>ETGQTLAANIWSDKTTAQNEPINLTNANAPIKNAKNLNSTITNVAAFDTKLNHLLVDTITGRVFVGGVNRLYQLSPDLELSETVKTGPQNDSVECSILDCPLNAVRSPTDNYNKVLLIDRATSRLIACGSLFQGTCTVRNLQNVSIIEHEVPDAVVANDANSSTVAFIAPGPPQHPVTNVMYVGVTYTNNSPYRSEIPAVASRSLEKTKMFQIASSAVTTGTRTFINSYARETYFVNYVYGFSSERFSYFLTTQLKHSHHSSPKEYITKLVRICQEDSNYYSYTEIPVECISDAQGGTKFNLVQAGFLGKPSSDLAQSLGISIQDDVLFAVFSKGEGNTPTNNSALCIYSLKSIRRKFMQNIKSCFNGSGMRGLDFISPSMPCVLTKLQTIGEDFCGLDVNSPLGGETPITSVPVAMFNTKLTSVAATSTSGYTVVFVGTSDGFLKKVVIESSSIANEYASFAVDLGSEINRDMQFDNQNLYIYVMSKTKVSKVKVFDCSDYKTCGDCLGARDPYCGWCSLENKCSPRSNCQDDANDPLYWVSYKTGKCTTITSVVPHQLQRTTARTLELIIDHLPQLKENLICAFTTEDKALFTNATKKRNGVNCTTPRTDMLPQIEQGKHHFTAKLSVRTRNGPDLVSTDFTFFDCSTHSSCTRCVSSEFPCDWCVEAHRCTHDTAENCRNDILVTGVSRIGPSYRSGPGFCPTGTKHHHHHH[2x];>ETGDVKPDLQTKQDKVLAHFIGNSTDYFKILDHNDEFVLVGAKDVIYNVSLNGLKEIARLEWHSTDADRELCALKGKHEWDCHNYLRVYALRPNGEVLLCGTNSYKPRCRHYTPVEVSSEEAGSAGHAHAMRYEVSRDVEAQGLCPYSPAHNSTYAFADGHLYSATVADFSGGDPLIYRENLRTEQYDLKQLNQPDFVGAIERNGYVLFFFRELSMEVMNFGKAVYSRVARVCKNDRGGPYSHGKSWTSFLKARLNCSVPGEFPFYFDEIQAISPIVESGSKSLIYAVFTTSVNAIPGSAVCAFNVDDILAAFDGEFKSQKDSQSHWLPVEREQVPKPRPGQCVEDSRTLTSIAVNFIKNHPLMEEAVPAVHGRPLLTKVNLHHRLTAIAVHPQVKSLSGAYYDVIYSGTDDGKVTKFINILSTHPNSTVDRLKTVVISEMQVLPLGTPIRELVISTSKNSLVVVSDGSLVSVPLHHCSHIVDCLGCLSLQDPICAWDLQTHECKNLATSQHKFGTKTYLQSLNSTKKAAALLCPHIPRDAPGAETVSFVTMAPPPTEEQKLLYSNVGSGTKHHHHHH[2x]

Semaphorin ligands interact with plexin receptors to contribute to functions in the development of myriad tissues including neurite guidance and synaptic organisation within the nervous system. Cell‐attached semaphorins interact in trans with plexins on opposing cells, but also in cis on the same cell. We have discovered a distinct mode of interaction through which the Drosophila semaphorin Sema1b and mouse Sema6A mediate binding in cis to their cognate plexin receptors. Sema1a and Sema1b are most closely related to the mammalian class 6 semaphorins and interact with the sole Drosophila class A plexin, PlexA.

John Wiley & Sons, LtdIn the crystal of 2:2 complex, two pairs of 1:1 complexes are packed together in the asymmetric unit with a relative orientation of 168.8° to form a pseudo tetramer. Each Sema1b molecule binds to both PlexA molecules in the pseudo tetramer. There are therefore two independent interaction sites, A and B, involving two different Sema1b‐PlexA orientations. The first, head‐to‐head orientation is equivalent to that observed in the 1:1 complex (interaction site A). In the second interaction mode, termed side‐on, Sema1b1‐2 and PlexA1‐4 bind through the site B or B’ with their carboxy‐terminal PSI domains oriented in parallel. While the B interaction site is extensive, the B’ interaction site is formed through distant contacts between three residues only. The structure of individual Sema1b1‐2 and PlexA1‐4 molecules in the 2:2 complex is very similar to those observed in the 1:1 complex, showing no significant conformational changes with the exception of the Exβ1‐β2 loop in the extrusion of Sema1b1‐2, which adopts a different orientation in order to avoid steric clashes with PlexA1‐4. In the side‐on orientation, the sema domains of Sema1b1‐2 and PlexA1‐4 are bound in a configuration in which the bottom face of PlexA1‐4 is oriented perpendicularly to the side edge of Sema1b1‐2. The most prominent, site 1, is formed by the extrusion of Sema1b and blade 6 of PlexA. The Exβ1‐β2 and β4B‐β4C loops are involved in semaphorin homodimerisation; however, for Sema1b1‐2 in the 2:2 complex these loops mediate interaction with PlexA suggesting that a B‐type interaction can only be mediated by a monomeric semaphorin molecule (Fig EV1H).>[4x]MQNEKLDHESVTQAMQPKDTPELRALYKSFEEESIIPLWTQLGDLMPIHPKSKAVPHVWKWSTLLRLARKSGELVPVGRGGERRALGLANPGLGGNAYISPTMWAGIQYLGPRETAPEHRHSQNAFRFVVEGEGVWTVVNGDPVRMSRGDLLLTPGWCFHGHMNDTDQPM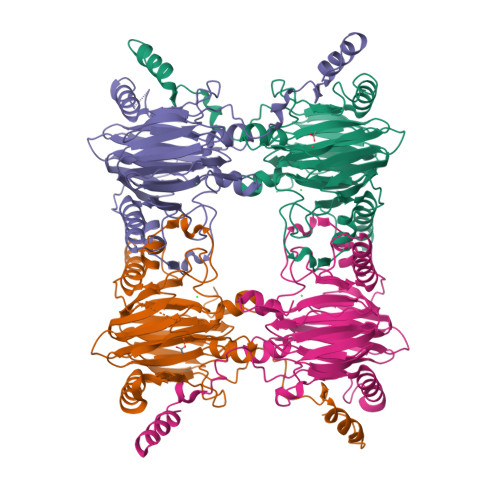AWIDGLDIPFSQQMDVGFFEFGSDRVTDYATPNFSRGERLWCHPGLRPLSGLQNTVASPIGAYRWEFTDRALTEQLLLEDEGQPATVAPGHAAIRYVNPTTGGDVMPTLRCEFHRLRAGTETATRNEVGSTVFQVFEGAGAVVMNGETTKLEKGDMFVVPSWVPWSLQAETQFDLFRFSDAPIMEALSFMRTKIEGQK> AATTQIGEIVKTVANTVESEIKAELGVIPSLNAVETGATSNTEPEEAIQTRTVINMHGTAECLVENFLGRSALVCMRSFEYKNHSTSTSSIQKNFFIWTLNTRELVQIRRKMELFTYLRFDTEITIVPTLRLFSSSNVSFSGLPNLTLQAMYVPTGARKPSSQDSFEWQSACNPSVFFKINDPPARLTIPFMSINSAYANFYDGFAGFEKKATVLYGINPANTMGNLCLRVVNSYQPVQYTLTVRVYMKPKHIKAWAPRAPRTMPYTNILNNNYAGRSAAPNAPTAIVSHRSTIKTMPNDINLTTA;> SPSAEACGYSDRVLQLKLGNSSIVTQEAANICCAYGEWPTYLPDNEAVAIDKPTQPETSTDRFYTLKSKKWESNSTGWWWKLPDALNQIGMFGQNVQYHYLYRSGFLCHVQCNATKFHQGTLLIVAIPEHQIGKKGTGTSASFAEVMKGAEGGVFEQPYLLDDGTSLACALVYPHQWINLRTNNSATIVLPWMNSAPMDFALRHNNWTLAVIPVCPLAGGTGNTNTYVPITISIAPMCAEYNGLRNAITQ;> GVPTCLLPGSNQFLTTDDHSSAPAFPDFSPTPEMHIPGQVHSMLEIVQIESMMEINNVNDASGVERLRVQISAQSDMDQLLFNIPLDIQLEGPLRNTLLGNISRYYTHWSGSLEMTFMFCGSFMTTGKLIICYTPPGGSSPTDRMQAMLATHVVWDFGLQSSITIIIPWISGSHYRMFNTDAKAINANVGYVTCFMQTNLVAPVGAADQCYIVGMVAAKKDFNLRLMRDSPDIGQSAILPEQA;> GAQVSRQQTGTHENANVATGGSSITYNQINFYKDSYAASASKQDFSQDPSKFTEPVAEALKAGAPVLK

Enterovirus 70 (EV70) is a human pathogen belonging to the family Picornaviridae. EV70 is transmitted by eye secretions and causes acute hemorrhagic conjunctivitis, a serious eye disease. The capsid of EV70 is composed of the subunits VP1, VP2, VP3, and VP4. The major capsid proteins of EV70 are organized with pseudo-T=3 icosahedral symmetry, with VP1 subunits forming pentamers around 5-fold symmetry axes and VP2 and VP3 subunits forming heterohexamers at 3-fold axes of the capsid.

Cryo-electron microscopy (cryo-EM) was used to determine a three-dimensional (3D) reconstruction of the virion of EV70 to a resolution of 2.63 Å. The nonenveloped capsid of EV70 has a diameter of 30 nm. The map enabled the building of the structure of capsid proteins except for residues 1 to 6 and 304 to 306 of VP1, 1 to 10 and 249 to 250 of VP2, and 1 to 27 and 60 to 68 of VP4. In contrast to EV-D68, the structure of which was solved using X-ray crystallography and cryo-EM, our reconstruction of EV70 enabled the building of the DE loop of VP1 that forms a protrusion around the 5-fold symmetry axes of the capsid. The lower local resolution of the cryo-EM map and higher-temperature factors of the atoms from the amino acids forming the BC and DE loops of VP1 indicate that they are flexible. In contrast, the pocket in VP1 of EV70 does not contain a continuous density corresponding to the pocket factor. In contrast, the pocket in EV70 VP1 is not completely collapsed, but the side chain of Met224 of VP1 partially blocks its central part. Thus, the discontinuous density fragments inside the pocket may correspond to solvent molecules. Whereas the main part of the EV70 pocket is formed by 26 residues of the VP1 subunit, the end of the pocket pointing toward the virion center is capped by residues from two VP3 subunits. Therefore, the pocket is accessible only from the outside of the virus particle.> SANEDMPVEKILEAELAVEPKTETYVEANMGLNPSSPNDPVTNICQAADKQLFTLVEWAKRIPHFSELPLDDQVILLRAGWNELLIASFSHRSIAVKDGILLATGLHVHRNSAHSAGVGAIFDRVLTELVSKMRDM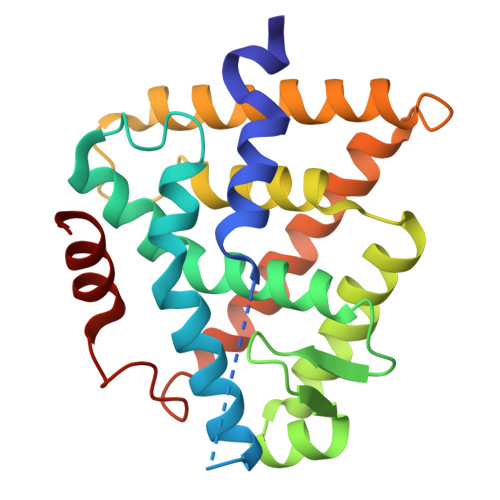QMDKTELGCLRAIVLFNPDSKGLSNPAEVEALREKVYASLEAYCKHKYPEQPGRFAKLLLRLPALRSIGLKCLEHLFFFKLIGDTPIDTFLMEMLEA>DNYRCPNPGDAFECFESDATARFCVSGKRGAYVICSKCRRKYEFCANGAKVSKRPEVECRADWASTECTSENSD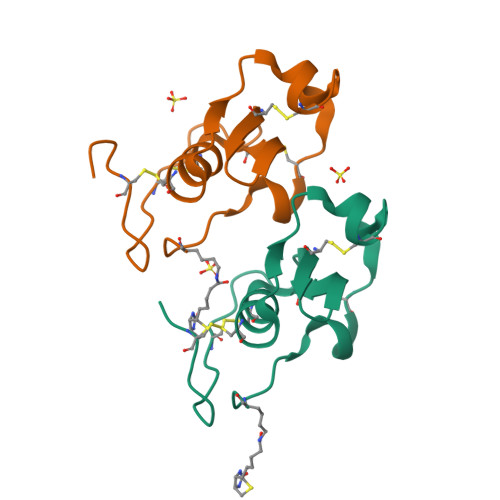VPSVMK[2x]>PRD[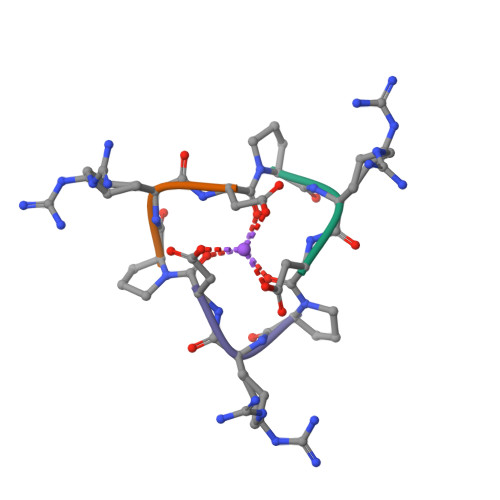2x]> ASSVNELENWSKWMQPIPDSIPLARISIPGTHDSGTFKLQNPIKQVWGMTQEYDFRYQMDHGARIFDIRGRLTDDNTIVLHHGPLYLYVTLHEFINEAKQFLKDNPSETIIMSLKKEYEDMKGAEDSFSSTFEKKYFVDPIFLKTEGNIKLGDARGKIVLLKRYSGSNEPGGYNNFYWPDNETFTTTVNQNANVTVQEKYKVSYDEKVKSIKDTMDETMNNSEDLNHLYINFTSLSSGGTAWNSPYYYASYINPEIANYIK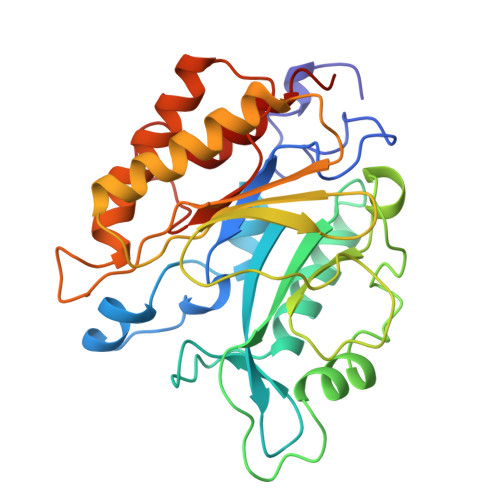QKNPARVGWVIQDYINEKWSPLLYQEVIRANKSLIKE> GPHMSYQVLARKWRPQTFADVVGQEHVLTALANGLSLGRIHHAYLFSGTRGVGKT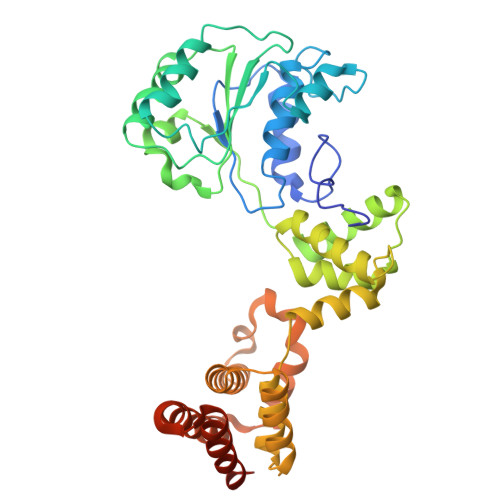SIARLLAKGLNCETGITATPCGVCDNCREIEQGRFVDLIEIDAASRTKVEDTRDLLDNVQYAPARGRFKVYLIDEVHMLSRHSFNALLKTLEEPPEHVKFLLATTDPQKLPVTILSRCLQFHLKALDVEQIRHQLEHILNEEHIAHEPRALQLLARAAEGSLRDALSLTDQAIASGDGQVSTQAVSAMLGTLDDDQALSLVEAMVEANGERVMALINEAAARGIEWEALLVEMLGLLHRIAMVQLSPAALGNDMAAIELRMRELARTIPPTDIQLYYQTLLIGRKELPYAPDRRMGVEMTLLRALAFHPRMPLPEPEVPRQ>[3x]GSAKDPHNHYIWAKLSAYHIAELLEQEKRYDESLAIIEEARVIWPNVPEFPLKKANILYVNHQLEDAKEIYQSLLENAAIDYQPIVLYEATNFMPHKMLGTIYLEEKDYTRAMTHFSKAYAENSSDYGVMFQMIMLLSKFHQPKEIFAFMERHHFISSTETGLRLLS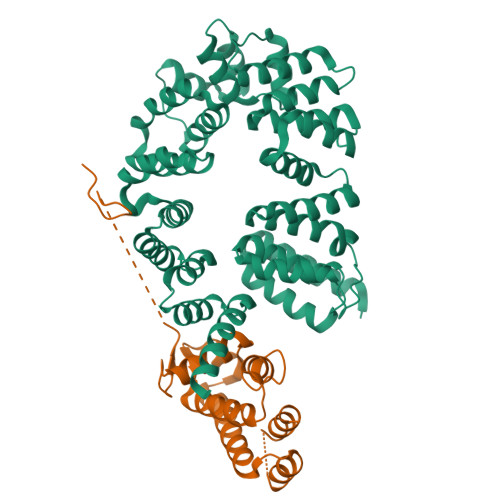MTTQQGYAELSELIVQSLTDVYPPVAEATEVKIATIRNVFPVISESAILFGIKEELIDAADLCLWHYENPQLPIENVMKNSDVGDIYDFIFENGPRISKKRYLFVLERAIALGKGEFADYLLALRNVYHDSINSHIADLFFQYDFADIALDFYNIVDADEVTKQGYINLINYLVDADVLDEALAIAERGIDNFSTDFRFYLWAIKIDTENRANRISEAMDEFPNNRYLAKLLDEVTMLQDTVTNNR;>[3x]GSAKDPMPKSEIRKLLQEIKKQVDNPGNSSTTEIKKMASEAGIDEQTAEEIYHLLTEFYQAVEEHGGIEKYMHSNISWLKIELELLSACYQIAILEDMKVLDISEMLSLNDLRIFPKTPSQLQNTYYKLKKELIQVEDIPKNKPGRKRKTQKNTKKEKTNIFGKVVPA> MVVDNFSKDDNLIELQTTSQYNPVIDTNISFYESDRGTGVLNFAVTKNNRPLSISSEHVKTFIVLKTDDYNVDRGAYISDELTIVDAINGRLQYVIPNEFLKHSGKVHAQAFFTQNGSDNVVVERQFSFNIENDLVSGFDGITKLVYIKSIQDTIEAVGKDFNQLKQNMADTQTLIAKVNDSATKGIQQIEIKQNEAIQAITATQTSATQAVTAEFDKIVEKEQAIFERVNEVEQQINGADLVKGNSTTNWQKSKLTDDYGKAIESYEQSIDSVLSAVNTSRIIHITSATD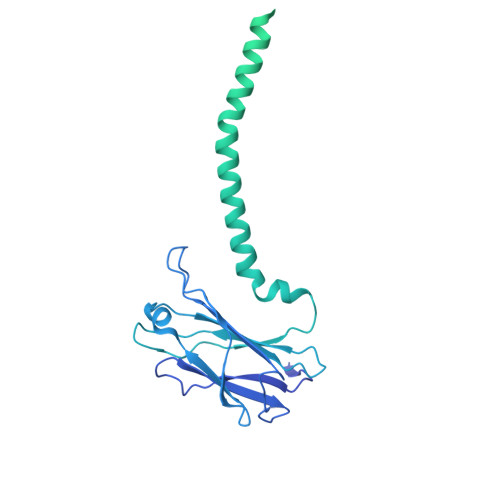APSFKDIGTVDTPKEDGVDDGSDIPVAPNTLGKSGVLVVYVVDDSTARATWYPDDSNDEYTKYKISGTWYPFYKKNDGDLTKQFVEETSNNALNQAKQYVDDKFGTTSWQQHKMTEANGQSIQVNLNNAQGDLGYLTAGNYYATRVPDLPGSVESYEGYLSVFVKDDTNKLFNFTPYNSKKIYTRSITNGRLEQQWTVPNEHKSTVLFDGGANGVGTTINLTEPYTNYSILLVSGTYPGGVIEGFGLTALPNAIQLSKANVVDSDGNGGGIYECLLSKTSSTTLRIDNDVYFDLGKTSGSGANANKVTITKIMGWK>MNHKVHHHHHHMGGGSTPLPLPQQQPPQQEPP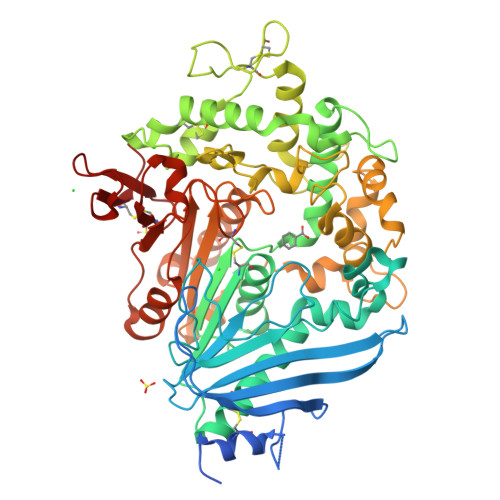PPPVPLASRAACEALKDGNGDMVWPNAATVVEVAAWRDAAPATASAAALPEHCEVSGAIAKRTGIDGYPYEIKFRLRMPAEWNGRFFMEGGSGTNGSLSAATGSIGGGQIASALSRNFATIATDGGHDNAVNDNPDALGTVAFGLDPQARLDMGYNSYDQVTQAGKAAVARFYGRAADKSYFIGCSEGGREGMMLSQRFPSHYDGIVAGAPGYQLPKAGISGAWTTQSLAPAAVGLDAQGVPLINKSFSDADLHLLSQAILGTCDALDGLADGIVDNYRACQAAFDPATAANPANGQALQCVGAKTADCLSPVQVTAIKRAMAGPVNSAGTPLYNRWAWDAGMSGLSGTTYNQGWRSWWLGSFNSSANNAQRVSGFSARSWLVDFATPPEPMPMTQVAARMMKFDFDIDPLKIWATSGQFTQSSMDWHGATSTDLAAFRDRGGKMILYHGMSDAAFSALDTADYYERLGAAMPGAAGFARLFLVPGMNHCSGGPGTDRFDMLTPLVAWVERGEAPDQISAWSGTPGYFGVAARTRPLCPYPQIARYKGSGDINTEANFACAAPP[6x]> GHMATGTRYAGKVVVVTGGGRGIGAGIVRAFVNSGARVVICDKDESGGRALEQELPGAVFILCD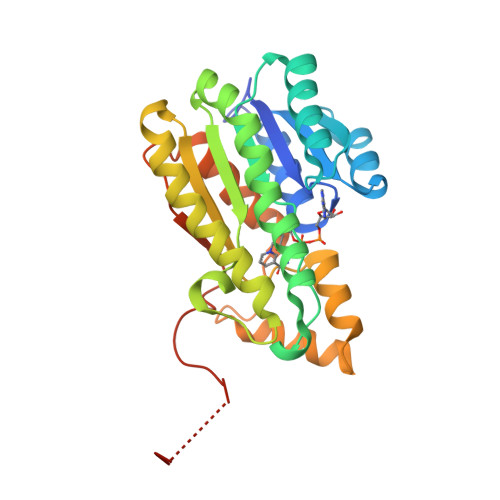VTQEDDVKTLVSETIRRFGRLDCVVNNAGHAPPPQRPEETSAQGFRQLLELNLLGTYTLTKLALPYLRKSQGNVINISSLVGAIGQAQAVPYVATKGAVTAMTKALALDESPYGVRVNCISPGNIWTPLWEELAALMPDPRASIREGMLAQPLGRMGQPAEVGAAAVFLASEANFCTGIELLVTGGAELGYGCKASRSTPVDAPDIPSGS> GAEFMDIDKDAFAAKEQALKQERPEGLVGGLQPKKLVNLENLVFDQGNHLMTNPRVRMPEGTTKRVFKGYEEIHVPPPKKRSDPTDQNIPVTELPEWARIPFNTTKTLNKIQSKCFPTAFLDDGNMLVCAPTGSGKTNVAMLTMLREIGKNRNEKGEIDLDAFKIVYIAPLKALVQEQVGNFGKRLEPYGIKVSELTGDRQLTKQQISETQVIVTTPEKWDVITRKATDISYTNLVRLIIIDEIHLLHDDRGPVLESIVSRTIRRTEQTGEPVRIIGLSATLPNYRDVASFLRVDFEKGLFYFDGSYRPCPLRQEFIGVTDKKAIKQLKTMNDITYQKVLEHVGQNRNQMLIFVHSRKETAKTAKYIRDKALEMDTINQILKHDAGTREVLQEAASSVNNTDLKDLLPYGFGIHHAGMSRADRTDVEDLFASGHIQ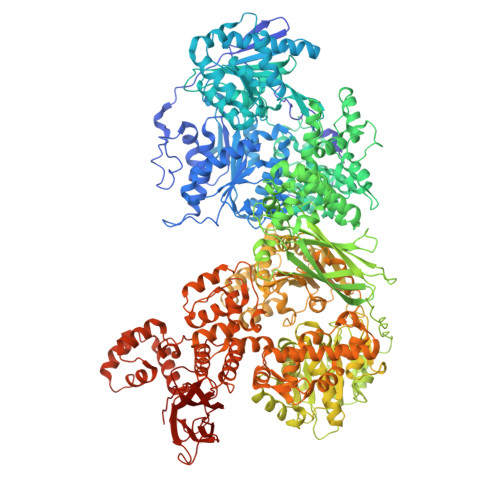VLVCTATLAWGVNLPAHTVIIKGTQVYSPEKGSWVELSPQDVLQMLGRAGRPQYDTYGEGIIITTQGEIPYYLSLLNQQLPIESQLVSKLVDSLNAEIVLGNVRNRDEGVEWLGYTYLFVRMLRSPGLYSVGAEYEDDVALEQKRVDLIHSAAMVLKKSNLIKYDEKTGKMQATELGRIASHYYISHESMDTYNKLIHPAMNDVELFRVFAQSGEFKYIPVRQEEKLELAKLLARVPIPVKESIEEPTAKINVLLQAYISRLKLEGLALMADMVYVTQSAGRILRAIFEICLKKGWASVAKLALNMCKMAEKRMWPTMSPLRQYPTCPAEIIKKAERMDVPWSSYFDLDPPRMGELLGMPKAGKTVCALVSKFPRVEIQGNVQPMTRSMLRIELTITPNFQWDVELHGVTESFWILVEDCDGEEILFHDVFILRKDLAEAEENEHTVEFTVPISEPMPPNYFISVISDRWMHSETRMPVSFQKLILPERFPPHTELLDLQPLPVSALKAKDYAALYPNWQQFNKIQTQTFNSLYNTDNNVLVAAPTGSGKTVCAEFALLRHWAKKDAGRAVYIAPFQELVDLRFQDWQKRLSHLRGGKEIVKLTGETTTDLKLLEQGDLILATPLQWDVLSRQWKRRKNVQTVELFIADDLHMLGGQMGYIYEIVVSRMHFIRTQTELPMRIVGLSVSLANARDIGEWIDAKKHDIYNFSPHVRPVPLELHIQSYTIPHFPSLMLAMAKPTYLAITQLSPDQPAIVFVPSRKQTRATARDLLTACLADDDEDRFLHVEVDQIRKLLDHVQEEALAEALSHGVGYYHEALSQSDKRIVKHLYNNGAIQVLIASRDVCWELDFTAHLVVVMGTQFFEGKEHRYIDYPLSEVLQMFGKALQPSKDGRSRGVLMLPAVKREYYKKFLNEALPVESHLHNFLPDAFVTEISTKMIESGEDAINWATFTYFYRRLLANPSYYGLQDPTHDGLSQYLSDLVETTLKQLSDARIIEMDEDEGTVAPLNAAMIAAYYNISYMTMEMFLLSLSHKSKLRTILEIVTAATEFESIQTRRHEEGILKRIYDHVPVKMNNPVWDSAHFKAFVLVQAHFSRMNLPIDLAKDQEVILQKILSLLSAIVDILSSEGHLNALNAMEMSQMVVQAMWDRDSPLKQIPNFTPEVVKVANKYGINDIFDFMEQMNPEENPNYASLVKDLGLTQAQLAQAANFTNNKYPDITLEFEVDDPDNIRAGEPAYLKIHIERELEEDEEFDPTVHAPFYPGKKSENWWLVVGEESTKTLLAIKRVTVGKELNVKLEFVVPSPGKHDLKLFLMSDSYVGVDQDPSFSVNVAEG> MSVKASGGSSLARPQLYQTVPVSAISQAEQQDRFLEGSELNELTAYFQSGALRLEIAETLTQNADLIVSRAANRIFTGGSPLSYLEKPVERQPALVGASSDSRNGSVTYAESNGSGGLFGGLRSVFSSTGPIPPGFRPINIARYGPSNMQKSLRDMSWFLRYTTYAIVAGDPNIIVVNTRGLKEVIENACSIDATIVAIQEMRAASADYFRNNAQAKEIVLQYFDILLSEFKAPTPANKVRQGPSNDIQGLELPQSYFNAAAKRQKYAMKPGLSALEKNAVIKAAYRQIFERDITKAYSQSISYLESQVRNGDISMKEFVRRLAKSPLYRKQFFEPFINSRALELAFRHILGRGPSSREEVQKYFSIVSSGGLPALVDALVDSQEYADYFGEETVPYLRGLGVEAQECRNWGMQQDLFSYSAPFRKVPQFITTFAQYDRPLPDQHVYGSGNDPLEIQFGAIFPKETRNPSKRPAPFNKDTKRILIHRGPAVNNQVGNPSAVGEFPGSLGAKVFRLNGGLPGAKVGKNTGTSVKFGESSTQALIRAAYRQVFGRDLYEGQRLSVAEIQLENGDISVREFIKRLAKSELFLKLYWAPHYVCKAIEYMHRRLLGRPTYGRQEMNQYFDIASKQGFYAVVEAMIDSKEYSDAFGEDTVPYERYLTPGGLQMRSARVGSLREDIGQRVDKEVTPRFVELGQVSAIRTEPEIAYRSNQGVTRQRQQTKVFKLVSTYDKVAVKNAIRAAYRQVFERDLEPYIINSEFTALESKLSNNEINVKEFIEGLGTSELYMKEFYAPYPNTKVIEMGTKHFLGRAPLNQKEIQQYNQILASQGLKAFIGAMVNGMEYLQTFGEDTVPYRRFPTLPAANFPNTERLYNKLTKQDKELVVPSFTPVVKVGG;> MPFTIDSARGIFPNTLAADVVPATIARFSQLNAEDQLALIWFAYLEMGKTLTIAAPGAASMQLAENALKEIQAMGPLQQTQAMCDLANRADTPLCRTYASWSPNIKLGFWYRLGELMEQGFVAPIPAGYQLSANANAVLATIQGLESGQQITVLRNAVVDMGFTAGKDGKRIAEPVVPPQDTASRTKVSIEGVTNATVLNYMDNLNANDFDTLIELFTSDGALQPPFQRPIVGKENVLRFFREECQNLKLIPERGVTEPAEDGFTQIKVTGKVQTPWFGGNVGMNIAWRFLLNPEGKIFFVAIDLLASPKELLNFAR;>MRMFRITACVPSQTRIRTQRELQNTYFTKLVPYDNWFREQQRIMKMGGKIVKVELATGRPGTNAGLA[2x];>[10x]MSIVTKSIVNADAEARYLSPGELDRIKAFVTGGAARLRIAETLTGSRETIVKQAGDRLFQKRPDIVSPGGNAYGEEMTATCLRDMDYYLRLVTYGVVSGDVTPIEEIGLVGVREMYRSLGTPIEAVAQSVREMKEVASGLMSSDDAAEASAYFDFVIGKMS;>MQDAITAVINSADVQGKYLDGAAMDKLKSYFASGELRVRAASVISANAATIVKEAVAKSLLYSDVTRPGGNMYTTRRYAACIRDLDYYLRYATYAMLAGDASILDERVLNGLKETYNSLGVPISSTVQAIQAIKEVTASLVGADAGKEMGVYLDYICSGLS[11x];> MALPLLNYAPKSQNVRVEGYEIGSEEKPVVFTTENILSSSDMDNLIEAAYRQIFFHAFKWDREKVLESQLRNGQITVRDFVRGLLLSNTFRNSFYEKNSNYRFVEHCVQKILGRDVYSEREKIAWSIVVATKGYQGLIDDLLNSDEYLNNFGYDTVPYQRRRNLPGREAGELPFNIKSPRYDAYHRRQLGFPQIVWQNEVRRFIPQEKKLTAGNPMNFLGMARSINPAANTIPKVSAQNINIEASVPRR;> MSVVSQVILQADDQLRYPTSGELKGIQAFLTTGAQRIRIAETLAENEKKIVDQAQKQLFKKHPEYRAPGGNAYGQRQYNQCLRDYGWYLRLVTYGVLAGNKEPIETTGLIGVKEMYNSLNVPVPGMVDAVTVLKDAALGLLSAEDANETAPYFDYIIQFMS;> MRDAVTTLIKNYDLTGRYLDRNAMDELKAYFESGSARIAAAAMINANSATIVKRAAAQLFEEIPELIRPSGNAYTTRRFSACLRDMDYYLRYASYALIAADNNVLDERVLQGLRETYNSLGVPIGPTVRGIQIMKEMIEAMAEDSSLNSTDFIASPFDHMTRELSELSV;> MLKKLFGAKKEFYVQLDESQAPAQVEEADVAIVKSEVAPVEKPAPTTSKKTSIKKKSATKAAAPVETPASAPVAPAPKAKVDPSQVAFASGDPIPQNVARRTPGPSLNRFKEMARQVKVKR

Cyanobacteria use large antenna complexes called phycobilisomes (PBSs) for light harvesting. However, intense light triggers non-photochemical quenching, where the orange carotenoid protein (OCP) binds to PBS, dissipating excess energy as heat. In these massive macromolecular assemblies, light-absorbing phycocyanobilin (PCB) pigments are covalently bound to phycobiliproteins that are tethered together by linker proteins and organized into the PBS rods and core cylinders. Using cryo–electron microscopy, we unveiled the OCP-PBS complex structure at 1.6- to 2.1-angstrom resolution, showcasing its inherent flexibility.

The newly obtained reconstruction recapitulates the known OCP-PBS structure, consisting of a tri-cylindrical core composed of Apc proteins with six emanating rods composed of Cpc proteins. On each side of the core, one OCP dimer is wedged between the top and bottom cylinders, as previously reported. The core of the OCP-PBS complex displays an overall slight twisting motion, with the top cylinder and bottom cylinders moving in opposite directions around the central symmetry axis. Our analysis also revealed that one of the B-cylinder’s ApcA/B hexamers is lost in a subset of particles. While this could occur during cryo-EM sample preparation, it agrees with previously reported sample instability or heterogeneity and may give rise to the presence of spectroscopically active components in PBS samples that are distinct from the holo-complex. The calculations using the high-resolution structure confirm that, to achieve an efficient quenching, there is no need to quench the lowest energy state emitting at 680 nm, which is associated with ApcD and ApcE subunits. Instead, quenching of ApcA pigments emitting at 660 nm is enough to provide photoprotection, as suggested in earlier reports based on analyses of time resolved fluorescence data.The enzyme, therefore, turned out to be scyllo-inositol dehydrogenase with L-glucose dehydrogenase activity (P. laeviglucosivorans scyllo-inositol dehydrogenase; Pl-scyllo-IDH). Further analysis showed that the enzyme oxidized L-glucose to L-glucono-1,5-lactone as the first step in the pathway for L-glucose metabolism. Pl-scyllo-IDH formed a homo-tetrameric structure in the asymmetric unit, and this structure was considered the biologically relevant form, since a similar unit has been observed for myo-IDH from B. subtilis and GFOR from Zymmomonas mobilis. The N-terminal domain adopted a Rossmann fold motif for the binding of NAD+, and the C-terminal domain bound substrate.

The apo-Pl-scyllo-IDH structure was refined at 1.75 Å, and the other complex structures ranged from 1.8–2.3 Å, depending on the substrate. Interestingly, in the apo structure, an acetate molecule originating from the crystallization solution was also found to be bound in the active site. This molecule formed hydrogen bonds with Y135, Y165, E195, and H318, which were the same residues used for substrate binding, other than the three catalytic residues, which suggests that these 4 residues may only be required for substrate binding, although the role of H318 remains unclear.

>MSNAEKALGVALIGTGFMGKCHAMAWRNVATAFGGLPPRLEVLADMPADKAHSLASSFGFARGTADWREAVSDPAVDVVSITTPNGLHREMAEAALAAGKHVWLEKPMALSVEDAQAMEAAARASDRRTIIGYNYTRSPAFRAAVDLIAEGAIGRPIHFRGMYDEDYMADPDLPWSWRLTRKDGGLGALGDLGCHLVSVMVSLMGPVARVYAQADTVITDRPHQGGTARVENEDQAQALIRFASGTSGEFSCSRVARGYRCRLAWEVQGTEGTLRFDQERMNELWLYQPGRPEIDGFRRILTGPAQPGFAAFCPGGGHNFGFNEQKVVEAEMLRQAIAGRGKAWPDFTDGLTIERVIHGMATSAQTGQPVNFLEHHHHHH[4x]>TKYSESYCDVLIVGAGPAGLMAARVLSEYVRQKPDLKVRIIDKRSTKVYNGQADGLQCRTLESLKNLGLADKILSEANDMSTIALYNPDENGHIRRTDRIPDTLPGISRYHQVVLHQGRIERHILDSIAEISDTRIKVERPLIPEKMEIDSS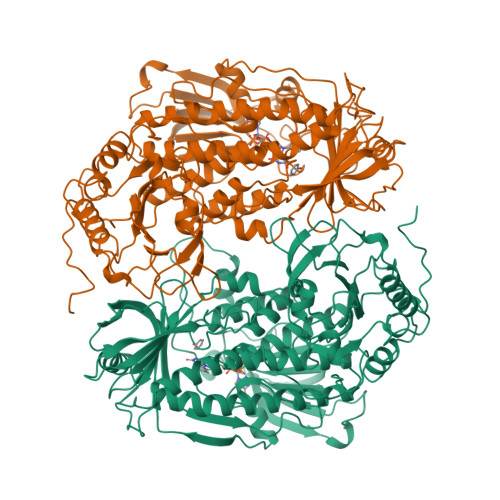KAEDPEAYPVTMTLRYMSDHESTPLQFGHKTENSLFHSNLQTQEEEDANYRLPEGKEAGEIETVHCKYVIGCDGGHSWVRRTLGFEMIGEQTDYIWGVLDAVPASNFPDIRSRCAIHSAESGSIMIIPRENNLVRFYVQLQARAEKGGRVDRTKFTPEVVIANAKKIFHPYTFDVQQLDWFTAYHIGQRVTEKFSKDERVFIAGDACHTHSPKAGQGMNTSMMDTYNLGWKLGLVLTGRAKRDILKTYEEERHAFAQALIDFDHQFSRLFSGRPAKDVADEMGVSMDVFKEAFVKGNEFASGTAINYDENLVTDKKSSKQELAKNCVVGTRFKSQPVVRHSEGLWMHFGDRLVTDGRFRIIVFAGKATDATQMSRIKKFSAYLDSENSVISLYTPKVSDRNSRIDVITIHSCHRDDIEMHDFPAPALHPKWQYDFIYADCDSWHHPHPKSYQAWGVDETKGAVVVVRPDGYTSLVTDLEGTAEIDRYFSGILVEPKEKSGAQTEADWTKSTA[4x]Heterologous expression in Streptomyces lividans TK21 and an in vivo analysis revealed that TleC catalyses the ‘reverse' prenylation of the cyclic dipeptide (−)-indolactam V (1) at the C-7 position of the indole ring with geranyl pyrophosphate (GPP) (C10) to produce lyngbyatoxin A (2), with the C19R configuration, as in the case of LtxC15. MpnD also catalyses the ‘reverse' prenylation of 1 at the C-7 position, with DMAPP (C5) to yield pendolmycin (3). The overall structures of TleC and MpnD adopt the ABBA-fold, which consists of ten antiparallel β-strands assembled into a circular β-barrel, surrounded by a ring of solvent-exposed α-helices, as observed in the structures of indole PTs and aromatic PTs222324252627. In contrast to typical indole PTs that exhibit broad substrate specificities towards the prenyl acceptors but with strict specificities towards the prenyl donors, it is remarkable that the indolactam-specific TleC and MpnD exhibited unusually relaxed substrate specificities towards the prenyl donors and accepted different chain lengths (from C5 to C25) of prenyl pyrophosphate in vitro.

To understand the intimate structural details of the enzyme reactions, we solved the X-ray crystal structures of TleC and MpnD as the apo structures (at 2.0 and 1.6 Å resolutions, respectively) and the ternary complexes with (−)-indolactam V and a DMAPP analogue dimethylallyl S-thiophosphate (DMSPP) (at 2.1 and 1.4 Å resolutions, respectively). Furthermore, the overall structures of TleC and MpnD are highly homologous to each other, with a root mean square deviation (RMSD) of 1.9 Å for the Cα-atoms. MpnD is also quite similar to these enzymes, with RMSD values of 2.9, 3.0 and 2.8 Å, respectively. In contrast, MpnD showed 109-fold higher activity for the C5 over the C10. In contrast, the rotation of the corresponding Tyr80 was not observed in the MpnD structures, because of the steric hindrance between Tyr80 and Met159. Moreover, the significant conformational differences of the loop between residues 166–174 in TleC and 152–160 in MpnD (RMSD of 1.9 Å for the Cα atoms), and the lack of a residue between 157 and 159 in MpnD (170 and 173 in TleC), result in the displacement of the Cα atom of the active site forming residue Met159 in MpnD by 1.3 Å towards the inside of the active site, as compared with Ala173 in TleC.

> MAGDPFVDNGTVSSQRPLRAVPGRYPPGATHLDAAVDTLVRCHAALGRAPSEAEAAVCLLRRLWGRWGNTPVERPGWRSYVAVDGSPFELSAAWNGDGPAEVRVTVEATADPPTPEGNQEAGWEYLRGLSRHPGAATARVLALEDLFRPQTPHDRCWIMHGMASRPGADPLFKVYLDPDARGAAEAPSVLDEAMDRLGVRAAWQGLRGWLDEHGGSGRIGSLALDLADTDDARVKVYVQHAGLDWADIDRQAAVARGHVPGAFSAALEEITGTEVPPHKPPVTCFAFHRGVGVPTAATLYIPMPAGVPESDARRRSAAFMRRSGLDSAAYLAFLAAATGDGEGVRALQNFVAYRPAAPGGRPRFACYVAPGLYRLEHHHHHH Here we investigated the aminopeptidase, P. aeruginosa aminopeptidase (PaAP) from P. aeruginosa, which is highly abundant in the biofilm matrix. PaAP is associated with biofilm development and contributes to nutrient recycling. We confirmed that post-translational processing was required for activation and PaAP is a promiscuous aminopeptidase acting on unstructured regions of peptides and proteins. PaAP contains an M28 Zn peptidase domain (residues 44–116 and 274–510) and a PA domain (residues 117–273).

We determined the elegant regulatory mechanism whereby the C-terminal propeptide region of PaAP binds in a groove between the protease and protease-associated (PA) domain, blocking access to the active site pocket. The structure of PaAP reveals the C-terminus binds in a groove between the PA and peptidase domains, which blocks access to the active site and locks these two domains into a closed conformation. The C-terminus is a propeptide sequence that binds between the PA and peptidase domains, inducing a closed inactive conformation where the active site is occluded. Although PaAP shows substantially increased activity after C-terminal tail removal, full-length protein is catalytic active, with lower kcat. Productive substrate binding to the closed conformation is unlikely given the active site and metal occlusion when C-terminal tail occupies the active site and inhibits PaAP. It is likely, therefore, that the full-length protein is sampling open (active, C-terminal tail away from the active site) and closed (inactive, C-terminal tail occupying the active site) conformations when free in solution.

> SEAQQFTEFWTPGKPNPSICKSPLLVSTPLGLPRCLQASNVVKRLQKLEDIASLNDGNRAAATPGYQASVDYVKQTLQKAGYKVSVQPFPFTAYYPKGPGSLSATVPQPVTYEWEKDFTYLSQTEAGDVTAKVVPVDLSLGAGNTSTSGCEAEDFANFPAGSIALIQRGTCNFEQKAENAAAAGAAGVIIFNQGNTDDRKGLENVTVGESYEGGIPVIFATYDNGVAWSQTPDLQLHLVVDVVRKKTETYNVVAETRRGNPNNVVMVGAHLDSVFEGPGINDNGSGSAAQLEMAVLLAKALPVNKVRFAWWGAAEAGLVGSTHYVQNLAPEEKKKIKAYLNFDMIGSPNFGNFIYDGDGSDFGLQGPPGSAAIERLFEAYFRLRGQQSEGTEIDFRSDYAEFFNSGIAFGGLFTGAEGLKTEEQAQKYGGTAGKAYDECYHSKCDGIANINQDALEIHSDAMAFVTSWLSLSTKVVDDEIAAAGQKLVPRGSQMQKSASQIERWGHDFIK>MRLLVGNDWSEELAEPTGSTGWAVQRLVWFARDGDVLVLPVAPQEEFLAYVTSLTGTRRSSLTVVVPPPGRLGAGALTADRLADPRFLAALREAFAGRPVHEVFALWPDAVVADLADALGCPEALEGHDFLTQSGGLIGSSKAAFRALAAGAGVALPAGAVCADRRRAHRHVTRLLDEGSPVILKQDYGSGSDGNEILSRTPGLALRGARALRVLADSAALDAYLDERWDWLTEGGRHRVVVERYHPGSRAYFAEFWISDGGVRLGGHGEMRYRPLPDSQ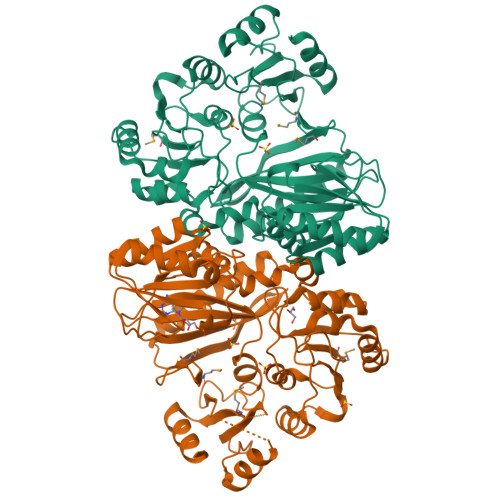VMPAPDLDQAQLDDLVEGGRRLCVALHALGYRGVLSADAVVTPAGEVLFTEHNGRATGSTHIYEIVGKRVVGPGFGTDRILLERVWPEGWEAPSFAGALTRLRDSGHLYDPETRRGAVILAAYNTHRKGVMLCYVAEDLEAALHREESVSRLFAPALSALEHHHHHH[4x]> 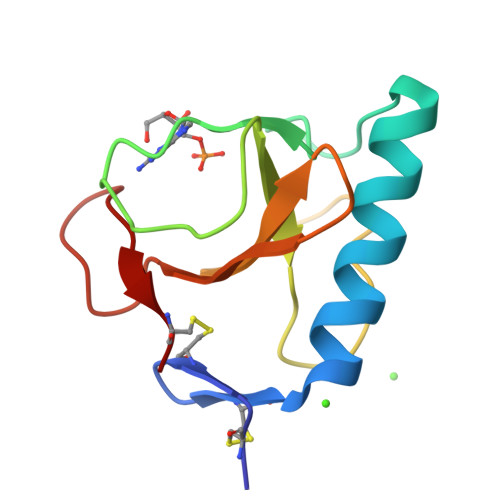ACDYTCGSNCYSSSDTSTAQAAGYKLHEDGETVGSNSYPHKYNNYEGFDFSVSSPYYEWPILSSGDVYSGGSPGADRVVFNENNQLAGVITHTGASGNNFVECT> MFEARLVQGSILKKVLEALKDLINEACWDISSSGVNLQSMDSSHVSLVQLTLRSEGFDTYRCDRNLAMGVNLTSMSKILKCAGNEDIITLRAEDNADTLALVFEAPNQEKVSDYEMKLMDLDVEQLGIPEQEYSCVVKMP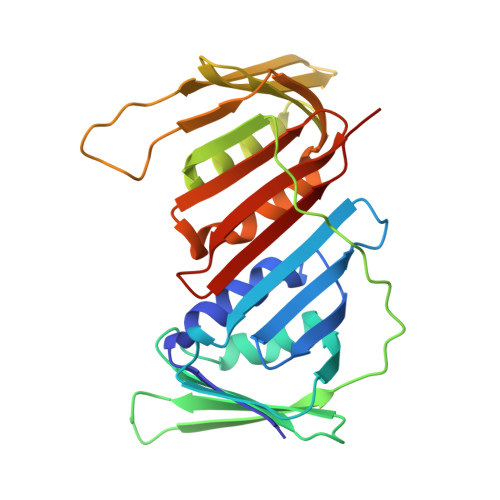SGEFARICRDLSHIGDAVVISCAKDGVKFSASGELGNGNIKLSQTSNVDKEEEAVTIEMNEPVQLTFALRYLNFFTKATPLSSTVTLSMSADVPLVVEYKIADMGHLKYYLAPKIEDEE> ARTVVLITGCSSGIGLHLAVRLASDPSQSFKVYAT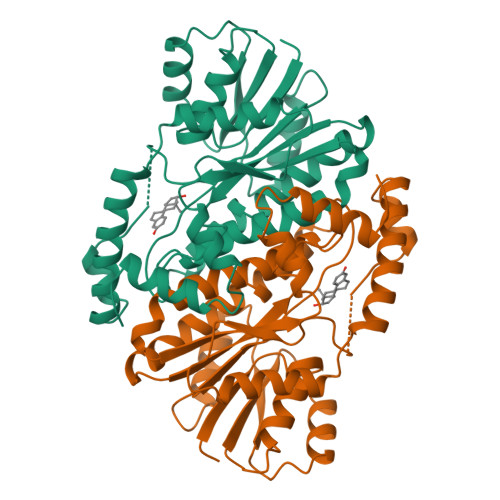LRDLKTQGRLWEAARALACPPGSLETLQLDVRDSKSVAAARERVTEGRVDVLVCNAGLGLLGPLEALGEDAVASVLDVNVVGTVRMLQAFLPDMKRRGSGRVLVTGSVGGLMGLPFNDVYCASKFALEGLCESLAVLLLPFGVHLSLIECGPVHTAFMEKVLGSPEEVLDRTDIHTFHRFYQYLAHSKQVFREAAQNPEEVAEVFLTALRAPKPTLRYFTTERFLPLLRMRLDDPSGSNYVTAMHREVFGDVPAKAEAGAEAGGGRGPGAEDEAGRSAVGDPELGDPPAAPQ The dual functions of TMEM16F as Ca2+-activated ion channel and lipid scramblase raise intriguing questions regarding their molecular basis. TMEM16 proteins form dimers; each subunit comprises 10 transmembrane helices (TMs) and contains its own ion conduction pore surrounded by TM3-TM7. Ca2+-dependent activation involves direct binding of Ca2+ ions to two contiguous Ca2+-binding sites formed by TM6-TM8. Here, we report evidence for a lipid scrambling pathway along a groove harboring a lipid trail outside the ion permeation pore.

To further investigate these lipid densities, we combined particles from all three States and carried out focused classification around this groove in a single monomer (See “Methods”). The particles clustered primarily to 2 classes that each contained approximately 40% of the particles and rendered 3.1 Å resolution structures. The overall protein organization of Class 1 and 2 is essentially indistinguishable. However, Class 1 almost entirely lacks lipid densities in the TM1-TM6 groove, whereas Class 2 has strong density for numerous lipids in this area. This indicates that our dataset contains a mixture of monomers in lipid-free and lipid-bound states, raising the intriguing possibility that the lipid trail aligns with the pathway for lipid scrambling.

>[2x]FEEFNGKPDSLFFTDGQRRIDFILVYEDESKKENNKKGTNEKQKRKRQAYESNLICHGLQLEATRSVSDDKLVFVKVHAPWEVLCYYAEIMHIKLPLKPNDLKTRSPFGNLNWFTKVLRVNESVIKPEQEFFTAPFEKSRMNDFYILDRDSFFNPATRSRIVYFILSRVKYQVMNNVNKFGINRLVSSGIYKAAFPLHDCRFNYESEDISCPSERYLLYREWAHPRSIYKKQPLDLIRKYYGEKIGIYFAWLGYYTQMLLLAAVVGVACFLYGYLDQDNCTWSKEVCDPDIGGQILMCPQCDRLCPFWRLNITCESSKKLCIFDSFGTLIFAVFMGVWVTLFLEFWKRRQAELEYEWDTVELQQEEQARPEYEAQCNHVVINEITQEEERIPFTTCGKCIRVTLCASAVFFWILLIIASVIGIIVYRLSVFIVFSTTLPKNPNGTDPIQKYLTPQMATSITASIISFIIIMILNTIYEKVAIMITNFELPRTQTDYENSLTMKMFLFQFVNYYSSCFYIAFFKGKFVGYPGDPVYLLGKYRSEECDPGGCLLELTTQLTIIMGGKAIWNNIQEVLLPWVMNLIGRYKRVSGSEKITPRWEQDYHLQPMGKLGLFYEYLEMIIQFGFVTLFVASFPLAPLLALVNNILEIRVDAWKLTTQFRRMVPEKAQDIGAWQPIMQGIAILAVVTNAMIIAFTSDMIPRLVYYWSFSIPPYGDHTYYTMDGYINNTLSVFNITDFKNTDKENPYIGLGNYTLCRYRDFRNPPGHPQEYKHNIYYWHVIAAKLAFIIVMEHIIYSVKFFISYAIPDVSKITKSKIKRE> GPGSMTTYTTIATSRPVAGVGLIRLDRPDALNALNQTLEAEVLDAARDFDADLEIGAIVVTGSERAFAAGADIAEMVTLTPHQARERNLLSGWDSLTQVRKPIVAAVAGYALGGGCELAMLCDLVIAADTARFGQPEI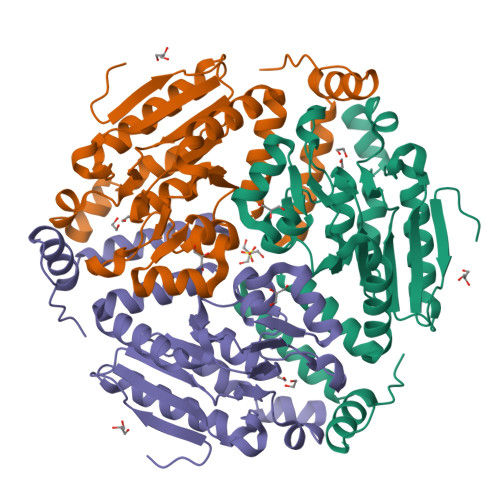TLGILPGLGGTQRLTRAVGKAKAMDLCLTGRSLTAEEAERVGLVSRIVPAADLLDEALAVAQRIARMSRPAGRAVKDAINEAFERPLSAGMRYERDAFYAMFDTHDQTEGMTAFLEKRTPEFTDR> GLPVMNTPGSNQFLTSDDFQSPSAMPQFDVTPELDIPGEVKNLMEIAEVDSVVPVNNVVGKLDTMDIFRIPVQSGNHQSTQVFGFQVQPGLDSVFKHTLLGEILNYYAHWSGSV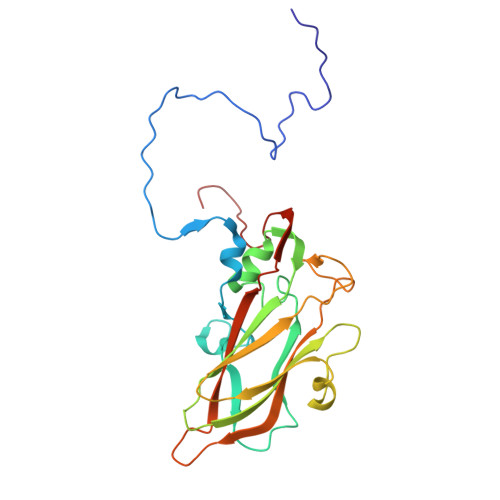KLTFVFCGSAMATGKFLLAYSPPGANAPKTRKDAMLGTHVIWDVGLQSSCVLCIPWISQTHYRLVHQDEYTSAGNVTCWYQTGIVVPAGTPTLCSIMCFVSACNDFSVRLLKDTPFIEQSALLQ> MFVYLSKRIAMPNGVKVTSIAWNDGQGWLACGGEKGLLKVLKVDGGPQGQRSGGLSSSQTLEGHDTTVDLVTWNQQYCKLTSSDVSGRIIVWVLHKGMWFEEMVNNRNSSRVVDFAWNPSGTKICITYEDGAVIVGGVDGNRYWGRELPYKLAKVCWGADGNSILFGTATGEVYVHDASSGEHLSQVEIKCNDGKAPSPLAGLSWHPAWVERPEPLATLAVCYQSGKLQLMTSIGDETPCNVDRDLPAHFISWNPSGTVLAVTAATPATEENGPGIVTQFFSTEGVHLRTLRVSGKQCGGITWEGGGLRVAIGVDSSVYFANVRPNYKYCYFKKTAVFAFTVPDKVEESVMFWNVNTNERRTKSVRGLQYMNACKDACVLISRPDTTQQQRMIQLVNAIGSPLETRFIDMELYTYDMNSSAVVCCGDESIYIWQFRDPSTAVDALDPISMQASRAESQERVIHVCDLVRGDTAPTMKVRSALTNDLISAMCVSETHMFVSLESGTLHVYQLSPLQLVSKYILFARAQSMSVNCNSTQLAVIHLGGITNVYCIEREKFSLVPCKADTIDGVELKDVWNLRWAVDDPHRFAVMEKTRMLVYNHGVAEEPVQSCANLCKFKSLKIRTLQLDELLLDPERPRKDYIVDFEAQLLRDMRAVLRDGTAKEAYEFAESHNTKKLWELLAEHTLFQLDFTYAEVAFIHCKDYAAIQFVKRVRSLDDPKKQLAEVNAYYRRFDEAERLYKDVDRKDLALDLRYRLGDWFGVVRLVQEGGGDEALLFQAWENIGDHYASRQKWSKAAQYYTQCRHYRKLARIFYIIEDYEMLTQLISMGEHDKELMVTLGNMLLTVGLAEEAAKAFIAANEPRMAVNGCVQVNMWNRAIALAK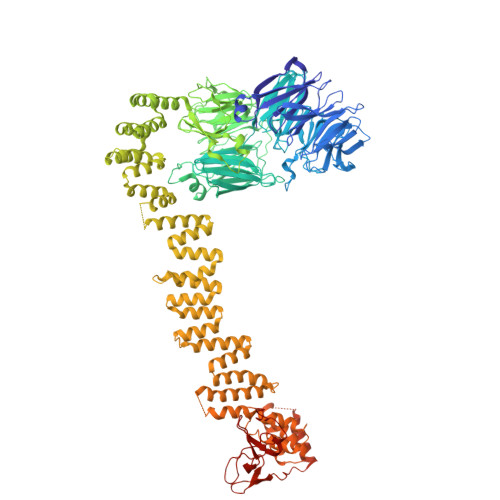EHRLEDVGQLLEKYAKYLIHRERLTEAIELYRKAGKHDEAATLLAQLGKRAALRDALKAKKFYVLSALEVQKYRTTAIALNRDGVAVVSEMLNKDRSTVSERTLDAAWRGAEAYHFLLMCQQQMADRNFKAALVLAMRLIEYDDLVAPVDGYSLIALTAYLVKNFGLCSKAFARLEQAERNDEAGGVAAAATTQLENFSLDLDVTHRTMASTCGGSTGGSTGMLSGGGGSALSGTTTSLQLTNPGKGVTRMAPMTYPTVSLRDPPRPFADLARHIFMTHSPVDTSVDSVPCPTCGSFNKEWAQRCIKCQQPFNTCIVSGCAIVSEDGAWQCSVCHRKALEAVVDKYRNCPLCHTPRKGRMRRGI Pent is a cationic (pI ∼ 8), designed β-propeller pentamer that binds one N-acetyl-d-glucosamine (GlcNAc) per monomer. Pentagonal proteins, which cannot adopt planar tessellations, are good candidates for forming pseudospherical enclosed arrangements such as dodecahedra or icosahedra. Synthetic macrocycles can mediate porous protein assemblies in the solid state, including cage-like structures (e.g., space group F432).14−17 The anionic sulfonato-calix[n]arenes (sclxn) are particularly useful mediators. Here, sclx8 directed the assembly of a pentameric β-propeller into a discrete icosahedral cage, evidenced in solution (i.e., a closed oligomer as opposed to an extended or infinite assembly occurring in the solid state).

Lys33, highly exposed on the Pent vertices, is located close to the 2- and 3-fold symmetry axes of the icosahedral assembly suggesting that the anionic calixarene can glue these sites. A crystal structure of Pent and the C6-symmetric sclx6 provides supporting evidence for this inference. Like the Pent–sclx8 cocrystals, Pent–sclx6 was cocrystallized in 1.2 M ammonium sulfate and 0.1 M sodium malonate pH 7. These crystals diffracted to 1.7 Å resolution, and the structure was solved in space group C2221 with an asymmetric unit comprising one Pent molecule. Four sclx6 ligands are evident in the unbiased electron density map. Adopting the “double partial cone” conformation, sclx6 binds the solvent exposed loop residues 30–34 at three of the Pent subunits. Consistent with our hypothesis, multiple noncovalent bonds are formed between the sulfonato-calixarene and up to 5 residues including Lys33 (and/or Lys22) from two protein subunits of two Pent molecules. The macrocycle position at the pentamer vertex suggests that sclx8 might form similar interactions in assembling the icosahedron. Potential calixarene binding sites were revealed in the Pent–sclx6 crystal structure, obtained under similar conditions.

>MSGFKFLFFSPDGTLYGVHNDKLYKGTPPTSDKDNWLARATLIGNGGW[5x]>[2x]MGFCLALAWTLLVGAWTPLGAQNPISWEVQRFDGWYNNLMEHRWGSKGSRLQRLVPASYADGVYQPLGEPHLPNPRDLSNTISRGPAGLASLRNRTVLGVFFGYHVLSDLVSVETPGCPAEFLNIRIPPGDPMFDPDQRGDVVLPFQRSRWDPETGRSPSNPRDPANQVTGW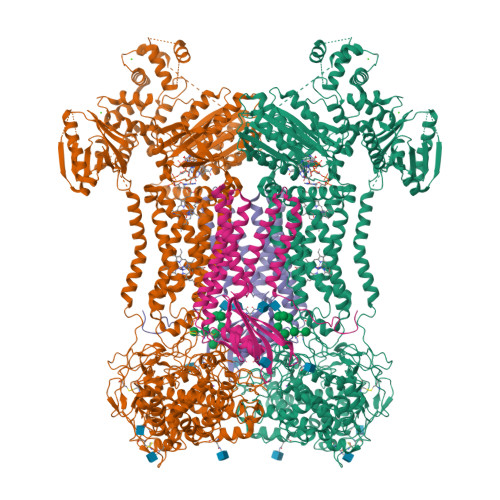LDGSAIYGSSHSWSDALRSFSRGQLASGPDPAFPRDSQNPLLMWAAPDPATGQNGPRGLYAFGAERGNREPFLQALGLLWFRYHNLWAQRLARQHPDWEDEELFQHARKRVIATYQNIAVYEWLPSFLQKTLPEYTGYRPFLDPSISSEFVAASEQFLSTMVPPGVYMRNASCHFQGVINRNSSVSRALRVCNSYWSREHPSLQSAEDVDALLLGMASQIAEREDHVLVEDVRDFWPGPLKFSRTDHLASCLQRGRDLGLPSYTKARAALGLSPITRWQDINPALSRSNDTVLEATAALYNQDLSWLELLPGGLLESHRDPGPLFSTIVLEQFVRLRDGDRYWFENTRNGLFSKKEIEEIRNTTLQDVLVAVINIDPSALQPNVFVWHKGDPCPQPRQLSTEGLPACAPSVVRDYFEGSGFGFGVTIGTLCCFPLVSLLSAWIVARLRMRNFKRLQGQDRQSIVSEKLVGGMEALEWQGHKEPCRPVLVYLQPGQIRVVDGRLTVLRTIQLQPPQKVNFVLSSNRGRRTLLLKIPKEYDLVLLFNLEEERQALVENLRGALKESGLSIQEWELREQELMRAAVTREQRRHLLETFFRHLFSQVLDINQADAGTLPLDSSQKVREALTCELSRAEFAESLGLKPQDMFVESMFSLADKDGNGYLSFREFLDILVVFMKGSPEEKSRLMFRMYDFDGNGLISKDEFIRMLRSFIEISNNCLSKAQLAEVVESMFRESGFQDKEELTWEDFHFMLRDHNSELRFTQLCVKGVEVPEVIKDLCRRASYISQDMICPSPRVSARCSRSDIETELTPQRLQCPMDTDPPQEIRRRFGKKVTSFQPLLFTEAHREKFQRSCLHQTVQQFKRFIENYRRHIGCVAVFYAIAGGLFLERAYYYAFAAHHTGITDTTRVGIILSRGTAASISFMFSYILLTMCRNLITFLRETFLNRYVPFDAAVDFHRLIASTAIVLTVLHSVGHVVNVYLFSISPLSVLSCLFPGLFHDDGSEFPQKYYWWFFQTVPGLTGVVLLLILAIMYVFASHHFRRRSFRGFWLTHHLYILLYVLLIIHGSFALIQLPRFHIFFLVPAIIYGGDKLVSLSRKKVEISVVKAELLPSGVTHLRFQRPQGFEYKSGQWVRIACLALGTTEYHPFTLTSAPHEDTLSLHIRAAGPWTTRLREIYSAPTGDRCARYPKLYLDGPFGEGHQEWHKFEVSVLVGGGIGVTPFASILKDLVFKSSVSCQVFCKKIYFIWVTRTQRQFEWLADIIREVEENDHQDLVSVHIYITQLAEKFDLRTTMLYICERHFQKVLNRSLFTGLRSITHFGRPPFEPFFNSLQEVHPQVRKIGVFSCGPPGMTKNVEKACQLINRQDRTHFSHHYENF;>[2x]MATLGHTFPFYAGPKPTFPMDTTLASIIMIFLTALATFIVILPGIRGKTRLFWLLRVVTSLFIGAAILAVNFSSEWSVGQVSTNTSYKAFSSEWISADIGLQVGLGGVNITLTGTPVQQLNETINYNEEFTWRLGENYAEEYAKALEKGLPDPVLYLAEKFTPRSPCGLYRQYRLAGHYTSAMLWVAFLCWLLANVMLSMPVLVYGGYMLLATGIFQLLALLFFSMATSLTSPCPLHLGASVLHTHHGPAFWITLTTGLLCVLLGLAMAVAHRMQPHRLKAFFNQSVDEDPMLEWSPEEGGLLSPRYRSMADSPKSQDIPLSEASSTKAYYRPRRLSLVPADVRGLAPAALSALPGALLAQAWRALLPGLRCPKAGKESRLGPPHSPWRFGPEGCEERWAEHTGDSPRPLRGRGTGRLWRWGSKERRACGVRAMLPRLVSNSGLKRPSCLDLPKCWDYRRDARAFFHLLEPTPCVTSRHTPLI>[3x]MHHHHHHENLYFQSMASGTTTTAVKIGIIGGTGLDDPEILEGRTEKYVDTPFGKPSDALILGKIKNVDCVLLARHGRQHTIMPSKVNYQANIWALKEEGCTHVIVTTACGSLREEIQPGDIVIIDQFIDRTTMRPQSFYDGSHSCARGVCHIPMAEPFCPKTREVLIETAKKLGLRCHSKGTMVTI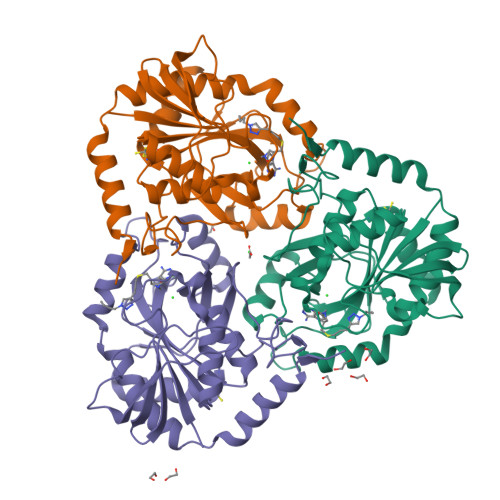EGPRFSSRAESFMFRTWGADVINMTTVPEVVLAKEAGICYASIAMATDYDCWKEHEEAVSVDRVLKTLKENANKAKSLLLTTIPQIGSTEWSETLHNLKNMAQFSVLLPRH>[4x]GSESEEVVSREVSGIKAAYEAELGDARKTLDSVAKERARLQLELSKVREEFKELKAR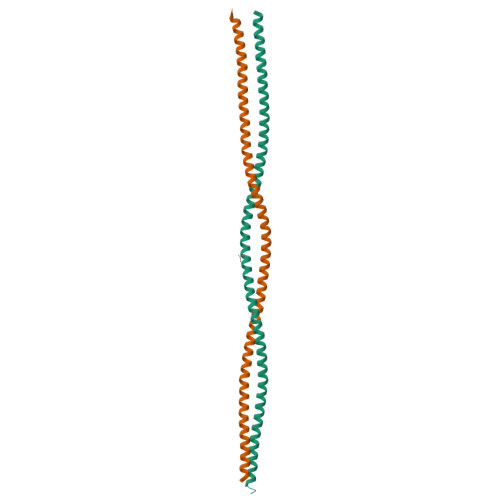NTKKEGDLIAAQARLKDLEALLNSKEAALSTALSEKRTLEGELHDLRGQVAKLEAALGEAKKQLQDEMLRRVDAENRLQTMKEELDFQKNIYSEELRETKRRH> EDQKDEKGYTDHDRKILQLCGELFDLDATSLQLKVLQYLQQETQATHCCLLLVSEDNLQLSCKVIGDKVLGEEVSFPLTMGRLGQVVEDKQCIQLKDLTSDDVQQLQNMLGCELQAMLCVPVISRATDQVVALACAFNKLGGDFFTDEDEHVIQHCFHYTGTVLTSTLAFQKE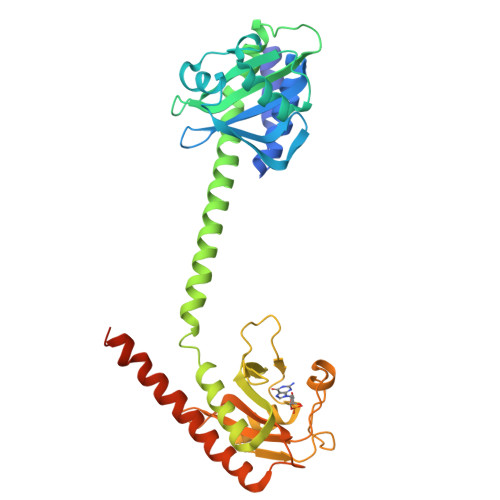QKLKCECQALLQVAKNLFTHLDDVSVLLQEIITEARNLSNAEICSVFLLDQNELVAKVFDGGVVDDESYEIRIPADQGIAGHVATTGQILNIPDAYAHPLFYRGVDDSTGFRTRNILCFPIKNENQEVIGVAELVNKINGPWFSKFDEDLATAFSIYCGISIAHSLLYKKVNEAQYRSHLANEMMMYLEHHHHHH>MSTRKAVIGYYFIPTNQINNYTETDTSVVPFPVSNITPAKAKQLTHINFSFLDINSNLECAWDPATNDAKARDVVNRLTALKAHNPSLRIMFSIGGWYYSNDLGVSHANYVNAVKTPASRAKFAQSCVRIMKDYGFDGVDIDWEYPQAAEVDGFIAALQEIRTLLNQQTITDGRQALPYQLTIAGAGGAFFLSRYYSKLAQIVAPLDYINLMTYDLAGPWEKVTNHQAALFGDAAGPTFYNALREANLGWSWEELTRAFPSPFSLTVDAAVQQHLMMEGVPSAKIVMGVPFYGRAFKGVSGGNGGQYSSHSTPGEDPYPSTDYWLVGCEECVRDKDPRIASYRQLEQMLQGNYGYQRLWNDKTKTPYLYHAQNGLFVTYDDAESFKYKA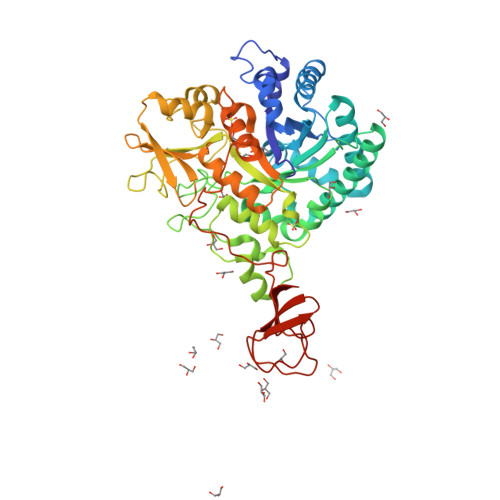KYIKQQQLGGVMFWHLGQDNRNGDLLAALDRYFNAADYDDSQLDMGTGLRYTGVGPGNLPIMTAPAYVPGTTYAQGALVSYQGYVWQTKWGYITSAPGSDSAWLKVGRVA[2x]> MQNSQDFSITELSLPKGGGAITGMGEALTPTGPDGMAALSLPLPISAGRGYAPAFTLNYNSGAGNSPFGLGWDCNVMTIRRRTHFGVPHYDETDTFLGPEGEVLVVADQPRDESTLQGINLGATFTVTGYRSRLESHFSRLEYWQPKTTGKTDFWLIYSPDGQVHLLGKSPQARISNPSQTTQTAQWLLEASVSSRGEQIYYQYRAEDDTGCEADEITHHLQATAQRYLHIVYYGNRTASETLPGLDGSAPSQADWLFYLVFDYGERSNNLKTPPAFSTTGSWLCRQDRFSRYEYGFEIRTRRLCRQVLMYHHLQALDSKITEHNGPTLVSRLILNYDESAIASTLVFVRRVGHEQDGNVVTLPPLELAYQDFSPRHHAHWQPMDVLANFNAIQRWQLVDLKGEGLPGLLYQDKGAWWYRSAQRLGEIGSDAVTWEKMQPLSVIPSLQSNASLVDINGDGQLDWVITGPGLRGYHSQRPDGSWTRFTPLNALPVEYTHPRAQLADLMGAGLSDLVLIGPKSVRLYANTRDGFAKGKDVVQSGEITLPVPGADPRKLVAFSDVLGSGQAHLVEVSATKVTCWPNLGRGRFGQPITLPGFSQPATEFNPAQVYLADLDGSGPTDLIYVHTNRLDIFLNKSGNGFAEPVTLRFPEGLRFDHTCQLQMADVQGLGVASLILSVPHMSPHHWRCDLTNMKPWLLNEMNNNMGVHHTLRYRSSSQFWLDEKAAALTTGQTPVCYLPFPIHTLWQTETEDEISGNKLVTTLRYARGAWDGREREFRGFGYVEQTDSHQLAQGNAPERTPPALTKNWYATGLPVIDNALSTEYWRDDQAFAGFSPRFTTWQDNKDVPLTPEDDNSRY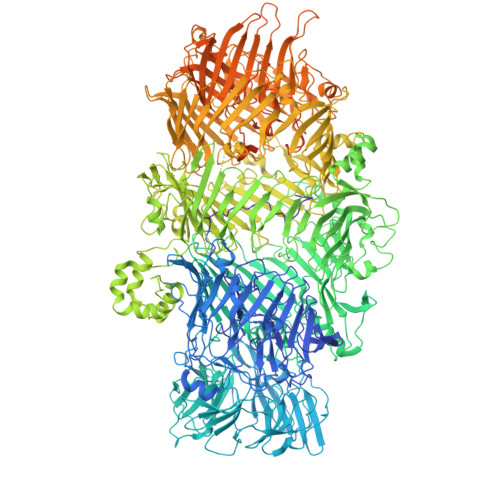WFNRALKGQLLRSELYGLDDSTNKHVPYTVTEFRSQVRRLQHTDSRYPVLWSSVVESRNYHYERIASDPQCSQNITLSSDRFGQPLKQLSVQYPRRQQPAINLYPDTLPDKLLANSYDDQQRQLRLTYQQSSWHHLTNNTVRVLGLPDSTRSDIFTYGAENVPAGGLNLELLSDKNSLIADDKPREYLGQQKTAYTDGQNTTPLQTPTRQALIAFTETTVFNQSTLSAFNGSIPSDKLSTTLEQAGYQQTNYLFPRTGEDKVWVAHHGYTDYGTAAQFWRPQKQSNTQLTGKITLIWDANYCVVVQTRDAAGLTTSAKYDWRFLTPVQLTDINDNQHLITLDALGRPITLRFWGTENGKMTGYSSPEKASFSPPSDVNAAIELKKPLPVAQCQVYAPESWMPVLSQKTFNRLAEQDWQKLYNARIITEDGRICTLAYRRWVQSQKAIPQLISLLNNGPRLPPHSLTLTTDRYDHDPEQQIRQQVVFSDGFGRLLQAAARHEAGMARQRNEDGSLIINVQHTENRWAVTGRTEYDNKGQPIRTYQPYFLNDWRYVSNDSARQEKEAYADTHVYDPIGREIKVITAKGWFRRTLFTPWFTVNEDENDTAAEVKKVKMPGSRPMKNIDPKLYQKTPTVSVYDNRGLIIRNIDFHRTTANGDPDTRITRHQYDIHGHLNQSIDPRLYEAKQTNNTIKPNFLWQYDLTGNPLCTESIDAGRTVTLNDIEGRPLLTVTATGVIQTRQYETSSLPGRLLSVAEQTPEEKTSRITERLIWAGNTEAEKDHNLAGQCVRHYDTAGVTRLESLSLTGTVLSQSSQLLIDTQEANWTGDNETVWQNMLADDIYTTLSTFDATGALLTQTDAKGNIQRLAYDVAGQLNGSWLTLKGQTEQVIIKSLTYSAAGQKLREEHGNDVITEYSYEPETQRLIGIKTRRPSDTKVLQDLRYEYDPVGNVISIRNDAEATRFWHNQKVMPENTYTYDSLYQLISATGREMANIGQQSHQFPSPALPSDNNTYTNYTRTYTYDRGGNLTKIQHSSPATQNNYTTNITVSNRSNRAVLSTLTEDPAQVDALFDAGGHQNTLISGQNLNWNTRGELQQVTLVKRDKGANDDREWYRYSGDGRRMLKINEQQASNNAQTQRVTYLPNLELRLTQNSTATTEDLQVITVGEAGRAQVRVLHWESGKPEDIDNNQLRYSYDNLIGSSQLELDSEGQIISEEEYYPYGGTALWAARNQTEASYKTIRYSGKERDATGLYYYGYRYYQPWIGRWLSSDPAGTIDGLNLYRMVRNNPVTLLDPDGLMPTIAERIAALKKNKVTDSAPSPANATNVAINIRPPVAPKPSLPKASTSSQPTTHPIGAANIKPTTSGSSIVAPLSPVGNKSTSEISLPESAQSSSSSTTSTNLQKKSFTLYRADNRSFEEMQSKFPEGFKAWTPLDTKMARQFASIFIGQKDTSNLPKETVKNISTWGAKPKLKDLSNYIKYTKDKSTVWVSTAINTEAGGQSSGAPLHKIDMDLYEFAIDGQKLNPLPEGRTKNMVPSLLLDTPQIETSSIIALNHGPVNDAEISFLTTIPLKNVKPHKR> GSSQKFSTSPSPTLDDGLDRIKCPKKHGMKLLRAFPKLNDTAGGTSDYGWGFWCDRCHKEVPALIKSKKRISKAQDERTHAPEENTFFYHCHCGYDLCKACGASIIHASNTLKENYSTELKNLAACFSTPS

Kinetoplastids are evolutionarily divergent eukaryotes that have an unconventional set of kinetochore proteins. In this study, we focused on KKT2 and KKT3, which are homologous to each other and have three domains conserved among kinetoplastids: A protein kinase domain classified as unique among known eukaryotic kinase subfamilies, a central domain of unknown function, and divergent polo boxes. In this report, we have revealed a unique zinc-binding domain in the KKT2 and KKT3 central domain, which is important for their kinetochore localization and function in T. brucei. In this study, we show that KKT2 and KKT3 are important for recruiting multiple kinetochore proteins, including KKT1, KKT4, KKT14, KKT22, and KKT23, while localization of KKT2 and KKT3 is independent from various kinetochore proteins. Together with the fact that KKT2 and KKT3 have DNA-binding motifs, these results support the hypothesis that KKT2 and KKT3 locate at the base of kinetoplastid kinetochores and play crucial roles in recruiting other kinetochore proteins.

Perkinsela is a highly divergent endosymbiotic kinetoplastid that lives inside Paramoeba. Our sequence alignment suggests that PkKKT2a and PkKKT2b have a CL-like domain but lack a C2H2 zinc finger. We determined the crystal structure of PkKKT2a551–679 at 2.9-Å resolution by Zn-SAD phasing, which confirmed the presence of a CL-like structure: Two β-sheets (residues 551–647), followed by an extended C-terminal α-helix (residues 648–679). The CL-like domain of PkKKT2a overlaps closely with that of BsKKT2 (RMSD: 0.79 Å across 39 Cα), with the exception of some differences being localized to the loop insertion and the absence of a C2H2 domain in PkKKT2a551–679, consistent with our sequence analysis. Taken together, our structures have revealed that the CL domain is conserved in BsKKT2 and PkKKT2a. Our fluorescence polarization assay showed that PkKKT2a551–679 has DNA-binding activity with a dissociation constant (Kd) of ∼500 nM on three DNA probes that have different GC contents (50 mer CEN is 50-bp DNA sequence from the CIR147 centromere repeat in T. brucei). To assess the importance of the CL domain for DNA binding, we next performed a fluorescence polarization assay for PkKKT2a551–679, which has mutations in zinc-coordinating residues (C646 and C649, corresponding to C616 and C619 in TbKKT2) and found that it has a similar DNA-binding affinity compared with WT PkKKT2a551–679. Taken together, these data have established that the CL domain is essential for the function of TbKKT2, which is consistent with the presence of CL, but not C2H2 zinc finger, in Perkinsela KKT2a.ADSL is involved in the de novo purine biosynthesis and recycling pathways in which it catalyses the conversion of 5-aminoimidazole-(N-succinylocarboxamide) (SAICAR) to 5-aminoimidazole-4-carboxamide ribotide (AICAR) and the conversion of succinyladenosine monophosphate (SAMP) to adenosine monophosphate (AMP), respectively. Both reactions are β-eliminations in which fumarate is released. Domain 1 (residues 22–112) and domain 2 form the base and one side of the active site thus creating a binding cleft for the substrate, while domain 3 (residues 365–450) resembles a lid which sits on top of the active site.

The apo structure of nADSL shows an identical tertiary and quaternary structure to that of hADSL, consisting of an all α-helical homotetramer that differs between the two variants with a RMSD (root mean square deviation) between Cα atoms of 0.5 Å. Structurally, domain 3 is the region which displays most of the structural differences between the apo forms of nADSL and hADSL when overlaying the tetrameric structures. However, this difference originates from small rigid body movements (of less than 1 Å) of the complete domain which can also be seen when overlaying the different protomers of nADSL (or hADSL) separately. A superposition of the separate domains 3 of nADSL and hADSL shows that the Ala429Val substitution has no effect on the local structure nor does it influence the local hydrogen bond networks. The SAXS curves from apo nADSL and hADSL are identical and fit well the theoretically calculated curves from the corresponding apo crystal structures (for q-values between 0.07 nm−1 and 4 nm−1). Hence, consistent with the results obtained by the structural comparison, nADSL and hADSL have an identical in-solution molecular structure in their apo state which is well described by their respective crystal structures.

>GSHMAAGGDHGSPDSYRSPLASRYASPEMCFVFSDRYKFRTWRQLWLWLAEAEQTLGLPITDEQIQEMKSNLENIDFKMAAEEEKRLRHDVMAHVHTFGHCCPKAAGIIHLGATSCYVGDNTDLIILRNALDLLLPKLARVISRLADFAKERASLPTLGFTHFQPAQLTTVGKRCCLWIQDLCMDLQNLKRVRDDLRFRGVKGTTGTQASFLQLFEGDDHKVEQLDKMVTEKAGFKRAFIITGQTYTRKVDIEVLSVLASLGASVHKICTDIRLLANLKEMEEPFEKQQIGSSAMPYKRNPMRSERCCSLARHLMTLVMDPLQTASVQWFERTLDDSANRRICLAEAFLTADTILNTLQNISEGLVVYPKVIERRIRQELPFMATENIIMAMVKAGGSRQDCHEKIRVLSQQAASVVKQEGGDNDLIERIQADAYFSPIHSQLDHLLDPSSFTGRASQQVQRFLEEEVYPLLKPYESVMKVKAELCL[4x]>[2x]EVVGGGDLGPNVLVFDPSTPDIQGKVDEVFRKQESNQFGTDRYALMFKPGTYNDINAQIGFYTSIAGLGLNPDDTTFNGDVTVDAGWFDGNATQNFWRSAENLALNPVNGTNRWAVSQAAPFRRMHVKGGLNLAPDGYGWASGGYIADSKIDGEVGPYSQQQWYTRDSSVGGWGNGVWNMTFSGVEGAPAQSFPEPPYTTLETTPVSREKPFLYLDGDDYKVFVPAKRTNARGTSWGNGTPEGESLPLDQFYVVKPGATAETINAAVDQGLHLLFTPGVYHVDQPIEIDRANTVAL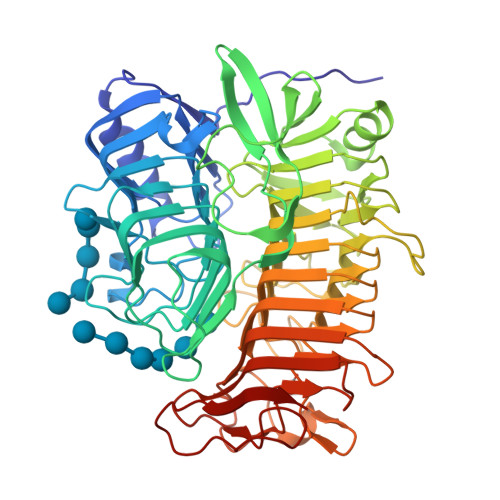GLGLATIIPDNGVTALKVGDVDGVKVAGLLVDAGPVNSETLVEVGSDGASGDHAANPTSLQDVFVRIGGAGPGKATTSIVVNSNDTIIDHTWVWRADHGEGVGWETNRADYGVHVKGDNVLATGLFVEHFNKYDVQWSGENGKTIFYQNAKAYDAPDQAAIQNGDIKGYAAYKVDDSVTTHEGWGMGSYCYFNVNPDIRQQHGFQAPVKPGVKFHDLLVVSLGGKGQYEHVINDIGDPTSGDTTIPSQVVSFP>[4x]MSAEREIPAEDSIKVVCRFRPLNDSEEKAGSKFVVKFPNNV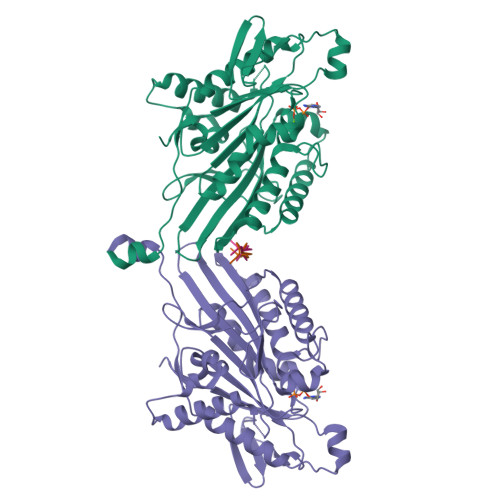EENCISIAGKVYLFDKVFKPNASQEKVYNEAAKSIVTDVLAGYNGTIFAYGQTSSGKTHTMEGVIGDSVKQGIIPRIVNDIFNHIYAMEVNLEFHIKVSYYEIYMDKIRDLLDVSKVNLSVHEDKNRVPYVKGATERFVSSPEDVFEVIEEGKSNRHIAVTNMNEHSSRSHSVFLINVKQENLENQKKLSGKLYLVDLAGSEKVSKTGAEGTVLDEAKNINKSLSALGNVISALADGNKTHIPYRDSKLTRILQESLGGNARTTIVICCSPASFNESETKSTLDFGRRAKTVKNVVCVNEELTAEEWKRRYEKEKEKNARLKGK;>[3x]GSGPQAQIAKPIRSGQGATS>MSLKGLRRLVLDVLKPHEPKTIVFALKLSELENVDGVNIHLSEIDQATENIKITILGNNLDYEQIKGVIEDMGGVIHSVDEVVAGKIIVESVEGHH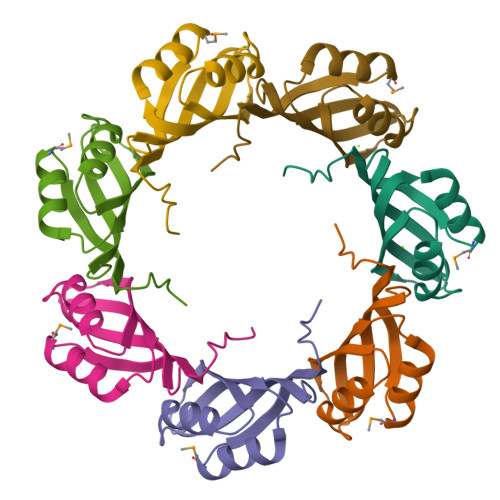HHHH[14x]>DDDLSARGSEERKPPVVEEDDVVGFDEEADIVINRLLGESNHLEVVPVVGMPGLGKTTLANKIYKHPKIGYEFFTRIWVYVSQSYRRRELFLNIISKFTRNTKQYHGMCEEDLADEIQEFLGKGGKYLVVLDDVWSDEAWERIKIAFPNNNKPNRVLLTTRDSKVAKQCNPIPHDLKFLTEDESWILLEKKVFHKDKCPPELVLSGKSIAKKCKGLPLAIVVIAGALIGKGKTPREWKQVDDSVSEHLINRDHPENCNKLVQMSYDRLPYDLKACFLYCSAFPGGFQIPAWKLIRLWIAEGFIQYKGHLSLECKGEDNLNDLINRNLVMVMERTSDGQIKTCRLHDMLHEFCRQEAMKEENLFQEIKLGSEQYFPGKRELSTYRRLCIHSSVLDFFSTKPSAEHVRSFLSFSSKKIEMPSADIPTIPKGFPLLRVLDVESINFSRFSREFYQLYHLRYVAFSSDSIKILPKLMGELWNIQTIIINTQQRTLDIQANIWNMERLRHLHTNSSAKLPVPVAPKNSKVTLVNQSLQTLSTIAPESCTEEVFARTPNLKKLGIRGKISVLLDNKSAASLKNVKRLEYLENLKLINDSSIQTSKLRLPPAYIFPTKLRKLTLLDTWLEWKDMSILGQLEHLEVLKMKENGFSGESWESTGGFCSLLVLWIERTNLVSWKASADDFPRLKHLVLICCDNLKEVPIALADIRSFQVMMLQNSTKTAAISARQIQAKKDNQTQQGTKNIAFKLSIFPPDL[2x]

Unlike most NLRs, the plant NLR required for cell death 2 (NRC2) belongs to a small NLR group characterized by constitutively high expression without self-activation. In this study, we discovered that SlNRC2 forms dimers and tetramers and higher-order oligomers at elevated concentrations. Using cryo-electron microscopy (cryo-EM), we performed structural analyses and found that SlNRC2 adopts an inactive conformation in both the dimeric and oligomeric states. Structural comparison shows that SlNRC2 dimerization and oligomerization act to stabilize the inactive conformation.

In contrast to the tetrameric and filamentous SlNRC2, the coiled-coil domains in the dimeric SlNRC2 were not well defined and hence were not included in the final refined model. The C2 symmetry-related SlNRC2 molecules in the dimer form a ‘head-to-head’ interaction through two interfaces. The first interface is facilitated by the packing of the N-terminal outer surface of the LRR domain from one protomer (SlNRC2A) against one end of the three-helix bundle of the NBD domain from the other protomer (SlNRC2B). This interface involves tight contacts of the C-terminal end of the α-helix from the second LRR of SlNRC2A with a short loop region which links α9 and α10 in SlNRC2B. Additionally, SlNRC2A Tyr506 from the loop region N-terminal to α22 interacts with SlNRC2B Glu271 and Arg275. The N-terminal end of the LRR domain of SlNRC2A symmetrically stacks with its equivalent from the SlNRC2B molecule, forming the second interface which mediates SlNRC2 dimerization. In the structure of the dimeric SlNRC2, the N-terminal end of the SlNRC2A LRR domain is wedged between the NBD and LRR domains of SlNRC2B, hence stabilizing the relative conformation of these two structural domains. A structural comparison between the inactive SlNRC2 dimer and a lateral dimer from the ZAR1 resistosome showed that the SlNRC2 dimerization interfaces overlap with the lateral dimeric ZAR1 surface mediating resistosome assembly. As IP6 was most prominently detected, this IP molecule was modelled in the extra cryo-EM density in the dimeric SlNRC2. On the other hand, these two LRR residues, along with the three residues from the WHD, directly interact with IP6/5 from the top. These interactions result in a total of 13 salt bridges and 4 hydrogen bonds between IP6 and SlNRC2.>MDFSRNLYDIGEQLDSEDLASLKFLSLDYIPQRKQEPIKDALMLFQRLQEKRMLEESNLSFLKELLFRINRLDLLITYLNTRKEEMERELQTPGRAQISAYRVMLYQISEEVSRSELRSFKALLQEEISKCKLDDDMNLLDIFIEMEKRVILGEGKLDILKRVCAQINKSLLKIINDYEEFSKERSS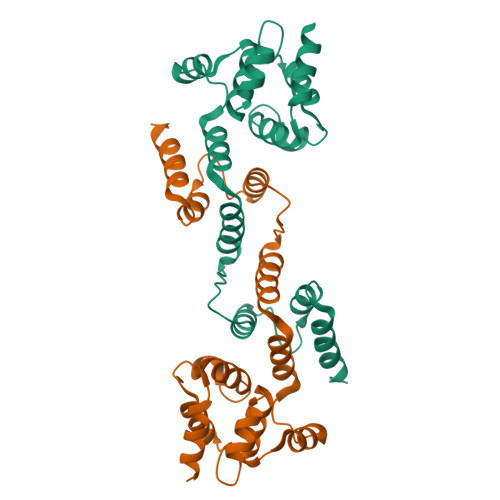S[4x]>MSRILVEDDNATPFHSMEIISSSLTLGQLLKNVSDVRKVEVGDETPVHEFFDRDGSSLDGDNDHLMRPVPFVLSFNNLTYNVSVRRKLDFHDLVPWRRTSFSKTKTLLDNISGETRDGEILAVLGASGSGKSTLIDALANRIAKGSLKGTVTLNGEALQSRMLKVISAYVMQDDLLFPMLTVEETLMFAAEFRLPRSLPKSKKKLRVQALIDQLGIRNAAKTIIGDEGHRGISGGERRRVSIGIDIIHDPIVLFLDEPTSGLDSTSAFMVVKVLKRIAESGSIIIMSIHQPSHRVLSLLDRLIFLSRGHTVFSGSPASLPSFFAGFGNPIPENENQTEFALDLIRELEGSAGGTRGLVEFNKKWQEMKKQSNPQTLTPPASPNPNLTLKEAISASISRGKLVSGGGGGSSVINHGGGTLAVPAFANPFWIEIKTLTRRSILNSRRQPELLGMRLATVIVTGFILATVFWRLDNSPKGVQERLGFFAFAMSTMFYTCADALPVFLQERYIFMRETAYNAYRRSSYVLSHAIVTFPSLIFLSLAFAVTTFWAVGLEGGLMGFLFYCLIILASFWSGSSFVTFLSGVVPHVMLGYTIVVAILAYFLLFSGFFINRDRIPQYWIWFHYLSLVKYPYEAVLQNEFSDPTECFVRGVQLFDNSPLGELTYGMKLRLLDSVSRSIGMRISSSTCLTTGADVLKQQGVTQLSKW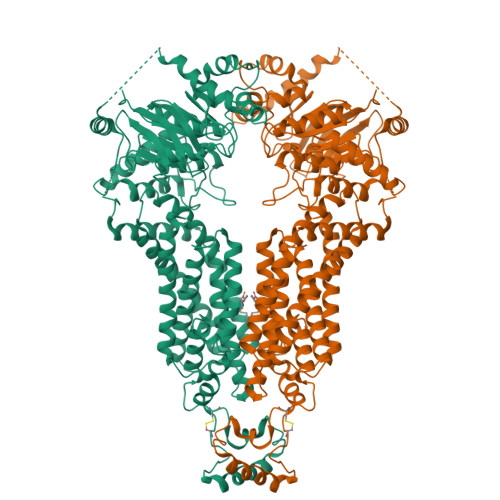NCLLITVGFGFLFRILFYLCLLLGSKNKRR[2x]>GSHVFKSRLQEYAQKYKLPTPVYEIVKEGPSHKSLFQSTVILDGVRYNSLPGFFNRKAAEQSAAEV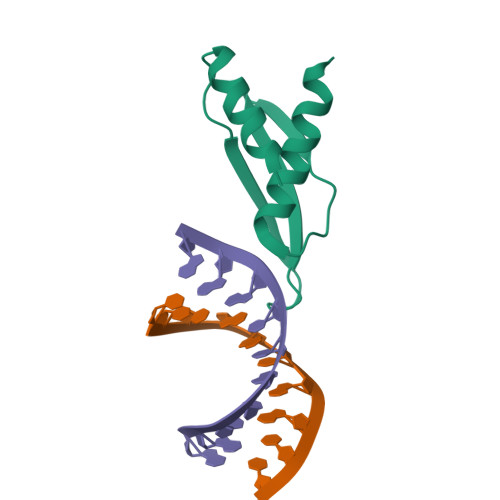ALRELAK[3x]>[2x]GGGRGRLILEHTLQGHKGRIWGVAWHPKGNVFASCGEDKAIRIWSLTGNTWSTKTILSDGHKRTIREIRWSPCGQYLASASFDATTAIWSKSSGEFECNATLEGHENEVKSVSWSRSGGLLATCSRDKSVWIWEVAGDDEFECAAVLNPHTQDVKRVVWHPTKDILASASYDNTIKMFAEEPIDNDWDCTATLTSHTSTVWGIDFDADGERLVSCSDDTTIKIWRAYHPGNTAGVATPDQQTVWKCVCTVSGQHSRAIYDVSWCKLTGLIATACGDDGIRIFKESSDSKPDEPTFEQITAEEGAHDQDVNSVQWNPVVAGQLISCSDDGTIKIWKVTE;>[2x]GGGRPTEIENINPNVYDRIKERVLTANEEDENVPDPFDKREIFDLIRNINDPEHPLTLEELHVVQEDLIRINDSQNSVHISFTPTIPHCSMATLIGLSIRVKLLRSLPPRFKVTVEITPGTHASELAVNKQLADKERVAAALENNHLAEVINQCIAAKG;>[2x]GGGRMAAATGLEEAVAPMGALCGLVQDFVMGQQEGPADQVAADVKSGGYTVLQVVEALGSSLENAEPRTRARGAQLLSQVLLQCHSLLSEKEVVHLILFYENRLKDHHLVVPSVLQGLRALSMSVALPPGLAVSVLKAIFQEVHVQSLLQVDRHTVFSIITNFMRSREEELKGLGADFTFGFIQVMDGEKDPRNLLLAFRIVHDLISKDYSLGPFVEELFEVTSCYFPIDFTPPPNDPYGIQREDLILSLRAVLASTPRFAEFLLPLLIEKVDSEILSAKLDSLQT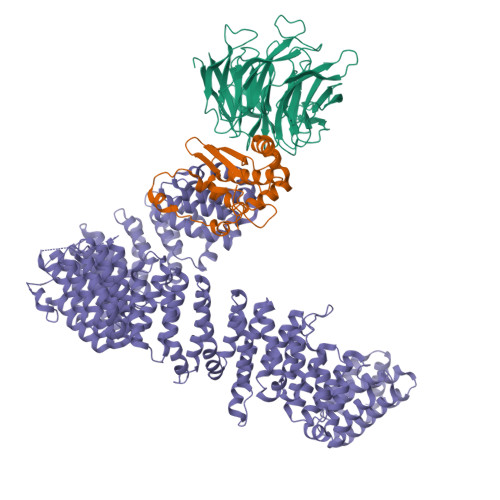LNACCAVYGQKELKDFLPSLWASIRREVFQTASERVEAEGLAALHSLTACLSCSVLRADAEDLLGSFLSNILQDCRHHLCEPDMKLVWPSAKLLQAAAGASARACEHLTSNVLPLLLEQFHKHSQSNQRRTILEMILGFLKLQQKWSYEDRDERPLSSFKDQLCSLVFMALTDPSTQLQLVGIRTLTVLGAQPGLLSAEDLELAVGHLYRLTFLEEDSQSCRVAALEASGTLATLYPGAFSRHLLPKLAEELHKGESDVARADGPTKCSRHFRCLQALSAVSTHPSIVKETLPLLLQHLCQANKGNMVTESSEVVAVCQSLQQVAEKCQQDPESYWYFHKTAVPCLFALAVQASMPEKESSVLRKVLLEDEVLAALASVIGTATTHLSPELAAQSVTCIVPLFLDGNTSFLPENSFPDQFQPFQDGSSGQRRLVALLTAFVCSLPRNVEIPQLNRLMRELLKQSCGHSCPFSSTAATKCFAGLLNKQPPGQQLEEFLQLAVGTVEAGLASESSRDQAFTLLLWVTKALVLRYHPLSACLTTRLMGLLSDPELGCAAADGFSLLMSDCTDVLTRAGHADVRIMFRQRFFTDNVPALVQGFHAAPQDVKPNYLKGLSHVLNRLPKPVLLPELPTLLSLLLEALSCPDSVVQLSTLSCLQPLLLEAPQIMSLHVDTLVTKFLNLSSSYSMAVRIAALQCMHALTRLPTSVLLPYKSQVIRALAKPLDDKKRLVRKEAVSARGEWFLLGSPGS> MDTHKVFVNRIINMRKIKLIGLDMDHTLIRYNSKNFESLVYDLVKERLAESFHYPEEIKKFKFNFDDAIRGLVIDSKNGNILKLSRYGAIRLSYHGTKQISFSDQKKIYRSIYVDLGDPNYMAIDTSFSIAFCILYGQLVDLKDTNPDKMPSYQAIAQDVQYCVDKVHSDGTLKNIIIKNLKKYVIREKEVVEGLKHFIRYGKKIFILTNSEYSYSKLLLDYALSPFLDKGEHWQGLFEFVITLANKPRFFYDNLRFLSVNPENGTMTNVHGPIVPGVYQGGNAKKFTEDLGVGGDEILYIGDHIYGDILRLKKDCNWRTALVVEELGEEIASQIRALPIEKKIGEAMAIKKELEQKYVDLCTRSIDESSQQYDQEIHDLQLQISTVDLQISRLLQEQN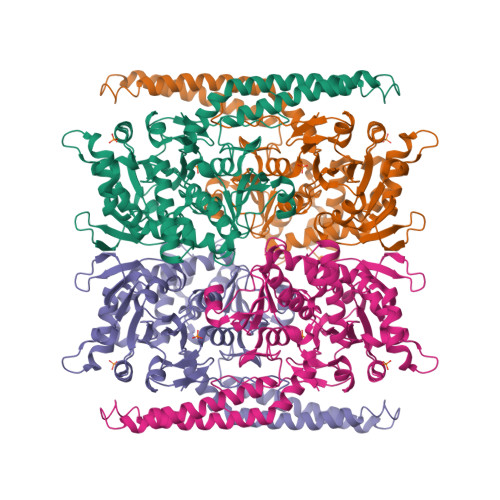SFYNPKWERVFRAGAEESYFAYQVDRFACIYMEKLSDLLEHSPMTYFRANRRLLAHDIDIAAALEHHHHHH The human AIP gene encodes a 37 kDa protein of 330 amino acids that, based on similarities to other proteins, is predicted to have an N-terminal immunophilin-like domain and a C-terminal tetratricopeptide repeat (TPR) domain. The TPR domain of AIP is similar to other TPR-domain proteins consisting of three pairs of anti-parallel helices and a Cα-7h. We present the structure showing the molecular interactions of the TPR domain of AIP in complex with the peptide-binding motifs of HSP90 and TOMM20. We found that the EDASRMEEVD (HSP90) and AQSLAEDDVE (TOMM20) peptides bind within the TPR-domain cleft and adopt a similar backbone conformation.

The structures show that the C-terminal carboxylate group and the C-terminal aspartate (HSP90) or glutamate (TOMM20) side-chain are involved in a series of hydrogen bonds that is reminiscent of the carboxylate clamp seen in the MEEVD-HOP complex. In the AIP-EDASRMEEVD (HSP90) structure the C-terminal carboxylic acid makes direct hydrogen bonds to one of the ring nitrogens of His 183 and to the amine nitrogen of Asn 187 and Asn 236. The C-terminal aspartic acid side-chain carboxyl-group also forms a direct interaction with the amine group of Lys 266. The valine side-chain is itself packed into a hydrophobic pocket formed by the side chains of Asn 187, Tyr 190, Arg 191 and Asn 236. The methionine of the HSP90 peptide is itself packed into a hydrophobic pocket formed by the side chains of Val 265, Lys 266, Phe 269, Lys 270 and Leu 298. The side-chain hydroxyl of Tyr 190 forms a direct interaction with the main-chain carbonyl of the second glutamate in the HSP90 peptide. In contrast, for the HSP90 peptide, Lys 266 forms direct hydrogen bonds with the carboxyl group of the shorter C-terminal aspartic acid side-chain as part of the carboxylate clamp. In contrast, in the HSP90 peptide bound structure Arg 304 is disordered and no significant interactions are made. The mode of interaction of these peptides resembles that of the HSP90 and HSP70 C-terminal peptides binding to the TPR-domain of CHIP rather than that of HOP. * 10-mer peptides were used in the crystallization, but only 6–7 resides were visible.

>[2x]AEEKAKAVPLIHQEGNRLYREGHVKEAAAKYYDAIACLKNLQMKEQPGSPEWIQLDQQITPLLLNYCQCKLVVEEYYEVLDHCSSILNKYDDNVKAYFKRGKAHAAVWNAQEAQADFAKVLELDPALAPVVSRELQALEARIRQ;>[2x]SRMEEVD> MSTLKQRKEDFVTGLNGGSITEINAVTSIALVTYISWNLLKNSNLMPPGISSVQYIIDFALNWVALLLSITIYASEPYLLNTLILLPCLLAFIYGKFTSSSKPSNPIYNKKKMITQRFQLEKKPYITAYRGGMLILTAIAILAVDFPIFPRRFAKVETWGTSLMDLGVGSFVFSNGIVSSRALLKNLSLKSKPSFLKNAFNALKSGGTLLFLGLLRLFFVKNLEYQEHVTEYGVHWNFFITLSLLPLVLTFIDPVTRMVPRCSIAIFISCIYEWLLLKDDRTLNFLILADRNCFFSANREGIFSFLGYCSIFLWGQNTGFYLLGNKPTLNNLYKPSTQDVVAASKKSSTWDYWTSVTPLSGLCIWSTIFLVISQLVFQYHPYSVSRRFANLPYTLWVITYNLLFLTGYCL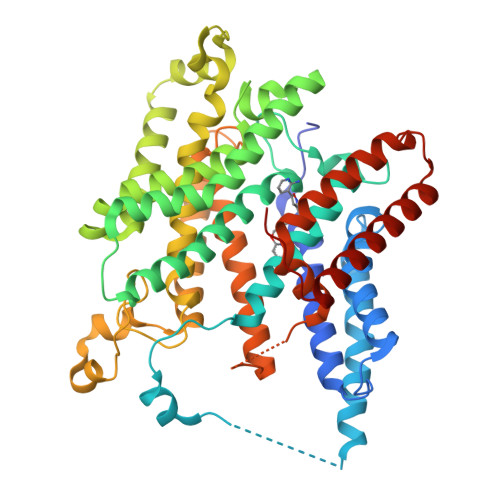TDKIFGNSSEYYKVAECLESINSNGLFLFLLANVSTGLVNMSMVTIDSSPLKSFLVLLAYCSFIAVISVFLYRKRIFIKL F-type ATP synthases are energy-converting membrane protein complexes that synthesize adenosine triphosphate (ATP) from ADP and inorganic phosphate. These universal enzymes function by using the energy stored in an electrochemical potential across the bioenergetic membrane by rotary catalysis. In mitochondria, F1Fo ATP synthase resides in the crista membrane where it is known to form dimers, which can further assemble into rows critical for inducing the membrane curvature and maintaining membrane potential and morphology. Here, we investigate the mechanism for the generation of the unique cristae in the Apicomplexa, using a combination of single-particle cryo-EM, cryo-ET and subtomogram averaging.

A large-scale preparation of T. gondii tachyzoite mitochondria and subsequent mild solubilisation with digitonin resulted in the isolation of intact ATP synthase complexes, which we identified as native hexamers. Masked refinement of the hexamer membrane region resulted in a 4.8-Å resolution map. Refining three copies of the dimer model into the hexamer map resulted in a good fit and showed that it forms a cyclic trimer of dimers. No additional subunits or substantial conformational changes of the dimer units were found in the hexameric assembly. The C2 symmetry axis through the dimer is tilted 22° with respect to the C3 axis in the hexamer, thereby bringing into proximity the lumenal regions, which extend 80 Å from the membrane. The hexamer model shows that each of the three dimer-dimer interfaces contributes ~1211 Å2 to hexamer contacts. Those contacts holding the hexamer together are found in two separate sites in the lumenal regions, which form a triangular subcomplex. In the first site, three copies of the subunit ATPTG9 are arranged around the C3-symmetry axis, directly beneath the central lipid bilayer. In the second site, located at the periphery of the lumenal region, ATPTG11 establishes a network of five interacting subunits. A helix hairpin of ATPTG11, containing a central cysteine pair, extends parallel to the membrane plane and mediates interactions between the dimers.

>[18x]MTIHSCLARRAVSVAASGARAFASGLGARAVAVGALQSARLLHTSSLRAAGAKISPSEMSRLLEERIAGWKTQTSTEEVGRVVSVGDGIARLFGLEGVQAGELVEFQNGMTGMALNLETDNVGVVIFGDDRSVLEGDSVKRTGRIVDVPIGPGLLGRVVDALGNPIDGKGPIPAKERRRVELKAPGIIPRKSVHEPMMTGLKCVDALVPVGRGQRELIIGDRQTGKTAVAVDAIINQKEINDSTDDESKKLYCIYVAVGQKRSTVAQIVKALEQRDAMKYTTVVAATASEAAPLQFLAPYSGCAMGEWFRDSGRHCVIIYDDLSKQATAYRQMSLLLRRPPGREAYPGDVFYLHSRLLERAAKMGDKSGGGSLTALPVIETQAGDVSAYIPTNVISITDGQIFLETELFYKGIRPAINVGLSVSRVGSAAQVKAMKQVAGTMKLELAQYREVAAFAQFGSDLDASTRQLLTRGTALTELLKQRQYSPMKNSVQVCVLYCGVKGYLDPLDPKEISRFESLFIDYINANHQDILKTIETEKELSEKTEAKLRAAVDEFVAMNEFKKK;>[6x]MQALRRGAAIPSRLLPRRDSWMSLAPFVAPNNAAAWRKLRDGAQEVQTVIERQSTPGKPQQIDWAKWESQIAHKDILNCLKTFYTNQVQILDRALGALETAKTPAPCEGAEKGWALFDAALSACAKSVEKSEELLSNGARALWVSCSNPPVWKVNTNEWLDSDQYWQAFVEKHHFYSQYQPGVVDPEAPQEVEAFKQAWHSRMGKFNDRSDTPMLYAYMNELPSWEYYDLHRSAFLEHMTYFLVRTGGDFRFFPEMPPWQWLAHMENLRFKLLSVAQSRRSQLQLANLERERALDFLPVDVEHHGEEYTQKFLQYETELFQACAARLMGHFMFLCDPFIPVQSAEALSAVTRVDNGKGKLFSLGDDVNALFYLPEQQRRDVERPTQAVQTLLGHLEATGRPFNPCYSELLHVHAEVLEERGEHWLTAPGECVSQAFLRRLRTDDPAYEVYCSYFKEMYERFAGAKEVSMEDGRKRLATIEKNAQEEAAAYGLALKTMGSAELAHKAREGAAKLEQLRKAQEKAAGKSAQTVQENKM;>[18x]MASPALQTCWRNLARLSGAQVRPSHFGAFSLGSRMSPFSSLLGARASPIATGRAGLRFLSSAAPNPGKKPASAAPPAGTNHGRITQVIGAVVDVHFDEQLPPILNSLEVQGHTNRLVLEVAQHLGENTVRTIAMDATEGLVRGQKVVDTGAPIQVPVGVETLGRIMNVIGEPVDECGPVPAKKTYSIHRAAPLFADQSTEPGLLQTGIKVVDLLAPYAKGGKIGLFGGAGVGKTVLIMELINNVANKHGGFSVFAGVGERTREGNDLYHEMMTTGVIKRKKLEDGKFDFTGSKAALVYGQMNEPPGARARVALTALSVAEYFRDEQGQDVLLFIDNIYRFTQAGSEVSALLGRIPSAVGYQPTLATDLGQLQERITTTKKGSITSVQAVYVPADDLTDPAPATTFAHLDATTVLSRQIAELGIYPAVDPLDSTSRMLAPEIVGQEHYDTARATQKLLQDYKSLQDIIAILGMDELSEEDKLVVSRARKIQRFLSQPFTVAEVFTGKPGRFVELPETIKSAQTILRGECDDLPEMAFYMCGGLEEVRSKAVKMAQEAASGK;>[6x]MNFSSSARWLAVRQSQTLGHTTRATVAAGRRVLAHSPAATEFTSFQSLHIGGDVCKLPLAVALGAAPSALGYGSAKHNQQRQYATLGSGWSFSKVQYTKYRITKPWTTDTTFDDIILSQPSKEDFAKFTKEAPLFLRFLKLVTDVEGRQEAFIQFAKRCENGLTVEKDVYVTKKELVDCLWKNGYTDTEINAFEIAFPADYKFHYPELAVLFDLTEEDCYKYCIRQRAATPEELVELKYTKPKNLVSSYGLCFLGVWFGLSNTVLSNAWFYSKTFPFGAVFYMLGSYFYRDIREKLWKEEKSLIHTAQENKNMGEESVYKQMKKYATDTKCLDYLSTFRTEVEDQIANYKVALVSQMRRQLTERLVEKLNGIQQAEKLIQGSLQDVMIREIVSSFKDLYKSRPELHDAAMQSAIQGLSGSDGAMDPVGAHFKASLQELAKVNLSTATADPMGTVVQRVAAVFQKREKEFLDTFTVKATEAQEIKTIVDKCHKGNTFDFHALSDEELRRLEQLYSTVNNRVGFETIHENSIKPVAPLSENSKGFVEFVNTQLEITKAKLRNARLTAFAHAFV;>[6x]MGGGGGGALNKLFPGYKDKIWMKVPVQWRQQMIQHWNKSYEKQVYSESVALNRTFQARNQLVLDRLKPSGAYRLPAVDYKRQLSRGTLVEGADFYLPTAQEQQRLARHFEPYSEQEQEERRKFRFQSISVYLAVALGASFVHDYFYQRRPVAWCLEKEPPHPPSYPFWFKSLFHSHDIPSVRRGYEVYRKVCATCHSMEQLHFRHLVGEVLPEKRVKQIAAEYDVTDGPNDQGEMYTRPGILGDAFPSPYPNEEAARYANGGAYPPDLSLITAARHFGPDYLMALLGGYRDPPEGVELRPGLYWNVWFPGNAIAMPPPLMDEMIDYEDGTPCNISQMSKDVVNFLTWATEPTADERKLYGLKCVSAIAIGTVLMTLWWRFYWAMYATRRIDFGKLKYL;>MSPVGRLFLGSKLPAQTWQSFRLQPALPQFAQKRFFSGGAAKPSWHVAREHRFGPTLPDHAYYGEHATYNYFVLFIRGMRPYLEKIFGDCASTIKNAAVAVYRPVNAFVVKHNPDLRLQFVAFASFIATHMAITKEFNDMYQRLVDITSLLELQAAQLHASEGFWDSESEQQEARLQRHAEHRNDLETTWEEALREATLARNFDVLVSYLNHGTSDGCGEHGACGHSGQNGIPPSVTWNFNAMPYGKENPDTKTFPIPDHEQPYRAFSLGFTANNLSGNWGDYIDRQDNKNALMRPARMMFTDVFIPTTK[6x];>MGEKQEEEGEEEKEGKGEGGGEGGREEEDEDGSAPVVSWLRIVEERECHEETDEAPETKIALPFSAQRSSRGFEARQVEVLVSANSAFLLSVLLASLFLSSSLPSFCPPRFLLSVLLALFKDKMAGDAPAAAAAPQQAGRTASASGVRTPGYLDLVGHSLKATSMDHGMQYSSIYWETSHRTYLPFWASLTQKFSWKIMDDQIRSFLRLPKPVTTEPFVFSSGSPYIRRYFGDADISVPVPLHAPAHFAFVPTGTVSPWEETGMETGPQGAAARGAAATAFRAVLESAWKCDIDEQIKEKLHSRAGAGAFHASGSTGGCPIPTDF[6x];>[6x]MALNRVPSRVLPFAVSGVYVHPRNACRLPAAAAVSSVPSSVSAFSSRTNFLSRSSSAVMSHPCAATARHFSFAIPPANAAALADPLPATPTPPPVFEAVSSASSGIASGTNALKNVEEVSTMERYEAAVYEESFKKPIVCLFFARFSLQSKVLLQPFLDFAASASNNATFFLIDCDRVPRAAYHARVENVPSLVVMKGDDAFRQTITDSVGVKTAGDLIQEARSALDQVLRLDQQEGGTKLQPGVSSYTHHIGVDNLNVYRKGWPVA;>[6x]MALPLLASRRLFSSFVFRGQPSTLSSNLSLVRIRGLHGGSLSPPSATLPRAVQLFSSRIAFSTAAAEDSGASQTLEGRYASALFRVAKKKNQLEKVYGDLESVRNALKDSSEFRLFVDSPAVSVQQKLDVLRQLVNRYKFDPLTGNLLTTLVENKRLPMLARVADAFDAMYRKEKGEVKCLVTSAKPLSAQQQKEIVAALQNRAGTQARLIIDYAVSPQIMGGLVVRLGEQVLDFSVATRLDRLQSQLLAPL;>[6x]MQNGVFTRENADFLVKSGADSPSSQSLLLRTSPSPLSLPRRRFIFLRSASVDLSERSSLACLAPFFCLASGVCLRSAFSLPFFARRGRPCLFFIFIFFFRVSFTANFRGKRVKMAASTIPISQWPSLLYAPPSSPANPAVEALPEMQFDDLHYPRQMLLCRGAGYSLEQCNRMAQPDARVTPENPAEKLLKEEAVAAIACLSQREGGKDEQCRYYIERMYKLANKEKQPEPGTLSKASTLACKLLGIHRPEA;>MFFSRLSLSALKAAPAREALPGLLSRQSFSSAGFSQFSSQKFFFSPSRNFSQSPLFQKHTPVHCNQRIASALVPTQQPAMTRQNPYAMQVGARYDAGVASLSAAIALMSVGGVAQGIGSLFAALVSGTARNPSIKEDLFTYTLIGMGFLEFLGIICVLMSAVLLYS[60x];>MAETREGGQSGAASILGAEAFPELLSKVPLNPQMDEDKHFNKYKWGNEPIPVNRRTGSRMNSSIYDNRNHEAVRHPWSTDARTFHPNDNPEADRINTQYSNMVSDSFPEGGFSDAPRFSSNWERLLAYHHGLYSPEKFNSTTKTADEIRLAVNDFAAKVHADDPKNACKYLMIEEFKCLQSAQARIDPQGAATKCVKWFNEWRQCAWDQEKMVKGYNYIEDRRARKHKPYIGAPDLQYS[6x];>[6x]MPSSSSEDAQGGNRFECVSNSTSPRRKNATKDEAACLQPRRSAVSGPREDVLCIRTTPQPHVRRGKSGPGRRKRMRFGRERERRDKKRGEGERKRTRFPFLRLHIEGGNANSRRPLCFPSRHSLLRNHYGSLSMAFRKVSPPKAPMSVFEARSSFLDLEQCARAAGPQRWEAECQGVRQRALQAAADVMSRECGAYGDSFFQCYRHGFRLEACQGEKATMQLLRCQRMVADRLVPL;>[6x]MGLSPAFAATAGCRLASPVANSSRFLSLLRLSRPRLNAAAPAAEAAKTLERNVPMKEILQPLWVVEPPNFLRQPVWKQFWEAQFANRSFFFFGNAWTSAAAFAFFIWWSRVFDPPPKERLDRYWLNSPKFRILSAFHNPGKRPGLKISLMTYEARYCYRGLDHPFTLNEMKDFLFKLREQYLVNKYEGIQFPFVFRQFNRVSTPGTLEVHTSPALQQQPHFHEEAAGHH;>MAAGSRFPFCTAARLSSRGTLPRLGEATFFAGAESQRSAGAFAKTLQRPFLRAPSTQLFPVGNRLGVSSARALVANAMEPRRFFAAAASAKATHALQPTGTGSVAFTRPGQGSNAQFQTSLADKTRGLLGVGFLRPTKMASFAATFLLNFRFYFMYMARTTFQAVRPLLAFSVFGEVMKLVLATMSSGLFSFLFSFVLAFEVFYFFLQCYISYTFLTMFFTVLF[6x];>MTALPPPPSANVAVSFTAAPAEPLSRGEVKAASLKLELQNIERELKDWWMSRKILRDRNIGLFNLLQHHNFAGLSVNNAKLSDSQRVMWTDLVQGKPDVEDKLSVDAREMKVDMYEKLFKQAADLENPCRMPGVAYLRCLRDTLTETQSARRSSCLNAFSSFDACRTGLLKQQSAAVENSLVRQNMADVRAKALFERRAVLLDLVEGK[6x];>MNTFFLTPAAAAARRVAVSFFARSSASGFPQHRVALRPFPSQRPAERAHNLAKSQTLRSVKAHGRQSGKKEQSTESGGRRGFRAAVGAGTGCMLAASPMLFTDYDNTASPKSELIFMAGNALGYCTERFFENEYGQSIFMFALGLAYLAMLGHEGKIHGAVWRMKHLFATNFKMVGHPRYAYALPKNPLLQDAAPTKTGSTSAKK[6x];>[6x]MSGDSVAPHQRAACEQLHSEYKQCLAKNGRTHFSACTDFHSKLRACENMLGTSYCIDEGINLMKCTKNPDPSFCAKEFVAMRECNRPQGPHLVLSSSPSSPPHYELRPEVKHLYNVDSTDLGSAVAPVRSKEQLDRVADSLKADLNLPGYGHIPYKWESLRPNPGA;>MAFAGAAAPLGVKGRSVFAGMRSFIGQRLGRLYDSFYYSQSSTKYVMVFLFPAGIFYTRFRADTKLGYHVFINEEKLYPDYSQNYFDTKWTNGRKVYLDDETTVEQLKAQIYGGKAAPENVKVACRGRVFEDADNVAMAVRAFCKRDPRLLLFQDNL[6x];>MSPPTASASVASSGSSPHMDRLLGDLKLLAAYDSAAGWQEPKAMESAFQSLSWDDADVLKALPQYLNCRGEQKRRVDFAYAALCPRPVDEKDPKQTLMSLWMKARLFSYDQKHPFVLSPFAATDKSTSAGAMTAEKPF[6x];>[6x]MVRNQRYPASPVQEIFLPEPVPFVQFDQTAPSPNSPPAPLPSPSLSQCEEQKDRYRDISSMFHRGVAGAEQVREAYNSMAKCFRRVSVAEVLESDPAFRQARNFTMDLKQAEDDQRYKQLQYGRVPSILTKYHL;>[6x]MLNFIPKRCPSVSLLFGKRPVQRIEVGQARHQLEIPVETIEKIYEGVDSRLEYHNKDYNAMKWKDFMKLKLDAYHLLEASQSETAAKSALSDLNWFSDLADIYSGQQTMAEMDVALKAQGEQKLSYPIQGKNIK;>MSWATRLLRMSSPRLGLLPLGRSVKLGGAKERVSFSQFFDSEYFWTKANVGPFFLFLFTSPFWYQGIKTVYASCRYRKLNEREIISDRYTWLHERMLEDEVERVLLEQVPAGGFDKTRPGLLLGPSTL[6x];>MPAPAASGAAAVLSKDIARSFRWMQAFAAVKGKPTAGSCAAGTAVVNPEDPTKVTLKGRYTNFSLQHIWEKYDYLQTHLLLRECMLSQVAKNPRLLDPEINAGLTPTVFMRVPPETQDPETQAKAAPQKGQAN[6x];>[6x]MATPPLQDGAPTNGGAATKPSCGARLQNFARMAIKGPSVPHSILFGVGAGCCAYAGYYLYRAMRLTFFDTESVALQSRLRYAEKQKLFHQELDRELAAGHIASLVAEYDPVATRLPFQPMQDRYRV;>MGFHFQQYIAMAGRAINPVQWTRAWRRMEGKSATEVYRDALAWTNNQFAQISRASQYRAWWWQNPLGMGLVLYGTYKAWHMIYMVRKQKKTAQLVAAAYGQGGQWLNPVPR[6x];>MPFMWRQRAYCAPVPSAFASQQPNGLGGEAGVRKPLLRSNSESLSVFSQIPDGLLGHTTSVTMGNSDIFFLPKPSNLLKIALPAFVFMPNLTIFTRAFPFYAHTSA[6x];>MSTSPGLAFANLTLLLDVPQLPAIWAVNAWRELNGLFTEMKTLAGTSDLLYPSNRYNPQNEKTNRMGRPRKYNHGEWMFGNSY[6x];>[6x]MFARAFSRFASLAAPAPQRGWNAFVLPSRHFATAAGGANPFKNQLLLTLSSPSEAIYVRTPVRSVTVPGSEGAMTMTNGHSQTVARLKAGEIIVRKGETGDEVERFFLSDGFVLFKSPEDDSGCCTAEVLGVEVVPVSMLDKESAATALQELLQQGAGATDEWTKARTLLGQELLSSVIRAAP;>MWRSSGVSFTRYASEMAALLRQCLKEPYRTQAMQRNQIHLKETVYQQGQVLTRETFNDIKKAFEAAAKHAGEK[6x];>MAGLASLSSVGALRGMRLVPAAHLLPLHSAFGQQTRNFGAGDLKIVAARMKSVKSIQKITKAMKMVAASKLRMDQRRLENGLPFATPVQKLVQRIPVDPKEKGTLAVLALSSDKGLCGGVNSFVAKQARIVIKENEMAGNAVQVYGVGDKIRSALQRTFGDRFKRIMTEVTRFPWNFGQACIIADRLMQDNPARLMVIYNHFKSAVAYDTLTLNVLTPTQAAQSAKEQLNTFEFEPEKTDVWKDLQDFYYACTVFGCMLDNIASEQSARMSAMDNASTNAGEMISSLTLRYNRARQAKITTELVEIISGANALE[6x];>MSSPCCVAIRRVARTTLESGRRQVDSKSTDVSPFFTGTQQMSLPSAGMVTKIRNFSSVKFMDQKRSGEETVYFKKEDEALLRNLLANHPEYDPKYSVDHMNAEVGSIARDITLACQKHGMKDPSAAFMKDLISIFGAHGYAKNSK[6x]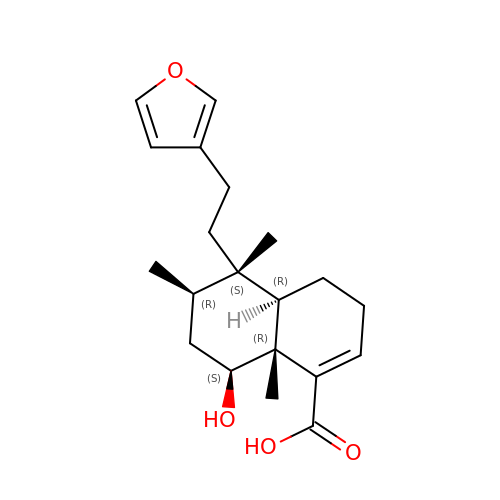(4~{a}~{R},5~{S},6~{R},8~{S},8~{a}~{R})-5-[2-(furan-3-yl)ethyl]-5,6,8~{a}-trimethyl-8-oxidanyl-3,4,4~{a},6,7,8-hexahydronaphthalene-1-carboxylic acid | C20 H28 O4 | XWKYXEIGWQYOCY-KWLVRGKZSA-N> MGVALGATRVIYPAGQKQEQLAVTNNDENSTYLIQSWVENADGVKDGRFIVTPPLFAMKGKKENTLRILDATNNQLPQDRESLFWMNVKAIPSMDKSKLTENTLQLAIISRIKLYYRPAKLALPPDQAAEKLRFRRSANSLTLINPTPYYLTVTELNAGTRVLENALVPPMGESTVKLPSDAGSNITYRTINDYGALTPKMTGVME;> DLYFNPRFLADDPQAVADLSRFENGQELPPGTYRVDIYLNNGYMATRDVTFNTGDSEQGIVPCLTRAQLASMGLNTASVAGMNLLADDACVPLTTMVQDATAHLDVGQQRLNLTIPQAFMSNRARGYIPPELWDPGINAGLLNYNFSGNSVQNRIGGNSHYAYLNLQSGLNIGAWRLRDNTTWSYNSSDRSSGSKNKWQHINTWLERDIIPLRSRLTLGDGYTQGDIFDGINFRGAQLASDDNMLPDSQRGFAPVIHGIARGTAQVTIKQNGYDIYNSTVPPGPFTINDIYAAGNSGDLQVTIKEADGSTQIFTVPYSSVPLLQREGHTRYSITAGEYRSGNAQQEKPRFFQSTLLHGLPAGWTIYGGTQLADRYRAFNFGIGKNMGALGALSVDMTQANSTLPDDSQHDGQSVRFLYNKSLNESGTNIQLVGYRYSTSGYFNFADTTYSRMNGYNIETQDGVIQVKPKFTDYYNLAYNKRGKLQLTVTQQLGRTSTLYLSGSHQTYWGTSNVDEQFQAGLNTAFEDINWTLSYSLTKNAWQKGRDQMLALNVNIPFSHWLRSDSKSQWRHASASYSMSHDLNGRMTNLAGVYGTLLEDNNLSYSVQTGYAGGGDGNSGSTGYATLNYRGGYGNANIGYSHSDDIKQLYYGVSGGVLAHANGVTLGQPLNDTVVLVKAPGAKDAKVENQTGVRTDWRGYAVLPYATEYRENRVALDTNTLADNVDLDNAVANVVPTRGAIVRAEFKARVGIKLLMTLTHNNKPLPFGAMVTSESSQSSGIVADNGQVYLSGMPLAGKVQVKWGEEENAHCVANYQLPPESQQQLLTQLSAECRLVPRGSWSHPQFEK;> ADSTITIRGYVRDNGCSVAAESTNFTVDLMENAAKQFNNIGATTPVVPFRILLSPCGNAVSAVKVGFTGVADSHNANLLALENTVSAASGLGIQLLNEQQNQIPLNAPSSALSWTTLTPGKPNTLNFYARLMATQVPVTAGHINATATFTLEYQ;> ADVTITVNGKVVAKPCTVSTTNATVDLGDLYSFSLMSAGAASAWHDVALELTNCPVGTSRVTASFSGAADSTGYYKNQGTAQNIQLELQDDSGNTLNTGATKTVQVDDSSQSAHFPLQVRALTVNGGATQGTIQAVISITYTYS;> FACKTANGTAIPIGGGSANVYVNLAPVVNVGQNLVVDLSTQIFCHNDYPETITDYVTLQRGSAYGGVLSNFSGTVKYSGSSYPFPTTSETPRVVYNSRTDKPWPVALYLTPVSSAGGVAIKAGSLIAVLILRQTNNYNSDDFQFVWNIYANNDVVVPTGGCDVSARDVTVTLPDYPGSVPIPLTVYCAKSQNLGYYLSGTTADAGNSIFTNTASFSPAQGVGVQLTRNGTIIPANNTVSLGAVGTSAVSLGLTANYARTGGQVTAGNVQSIIGVTFVYQ

Uropathogenic Escherichia coli strains use filamentous type 1 pili to adhere to and invade uroepithelial cells. The pilus consists of a flexible tip fibrillum, formed by the adhesin FimH and the subunits FimG and FimF. The pilus rod is a helical assembly of up to 3000 copies of the main subunit FimA, terminated by a single copy of the subunit FimI that anchors the rod to the assembly platform FimD in the outer membrane. The assembly platform FimD in the outer membrane of uropathogenic E. coli is the catalyst of type 1 pilus assembly.

As a consequence of the fact that incorporation of the first FimA subunit is rate limiting for pilus rod assembly, we obtained a mixture of FimD-rod complexes and FimDHGFC complexes that had not yet incorporated a single FimA after completion of FimD-catalyzed tip assembly. In conformer 1, the structure closely resembles PDB-ID 6E1522, with the NTD remaining unoccupied. However, the resolution did not allow unambiguous assignment of the incorporated subunits. The FimD-rod and FimDHGFC structures provide further insight into pilus assembly and suggest that FimD quickly adopts the post-handover conformation on the periplasmic side, driven by quaternary structure formation of the pilus rod on the extracellular side.4-[[(3S)-3-cyclopropyl-2-azaspiro[3.3]heptan-2-yl]methyl]-N-[[(3S)-3-oxidanyl-1-[6-[(phenylmethyl)amino]pyrimidin-4-yl]piperidin-3-yl]methyl]benzamide 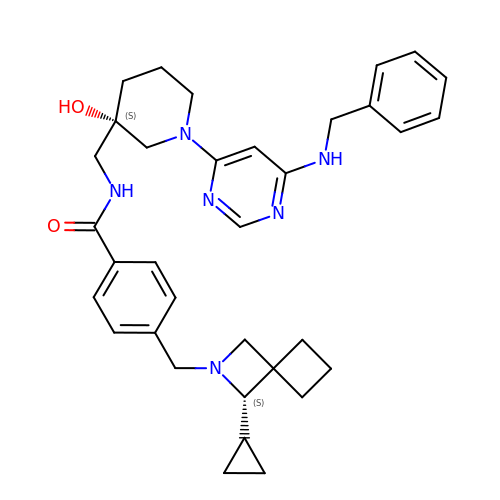| C34 H42 N6 O2 | OWDBESCKAVDZRB-VBTAUBHQSA-N Cohesin, a ring-shaped protein complex that wraps around sister chromatids is the molecular agent of sister chromatid cohesion, which persists from the time of DNA replication until anaphase. A distinct protein complex containing Scc2NIPBL and Scc4Mau2 (Scc2/4) initiates linkage of cohesin with DNA, and an in vitro reconstitution of cohesin loading by Scc2/4 suggests that the product of this reaction is a topological protein–DNA linkage. In addition to initiating a connection between cohesin and chromatin, Scc2/4 determines the timing and location of cohesin loading. We report here the structure of yeast Scc4 in complex with an N-terminal fragment of Scc2 and demonstrate that Scc4 determines cohesin localization through a conserved patch on its surface.

We obtained crystals of full-length Scc4 in complex with an N-terminal, 181-residue fragment of Scc2. We used an incomplete model, built into a 2.8 Å resolution map, to obtain phase information by molecular replacement for diffraction data from crystals of a native protein complex, extending to a minimum Bragg spacing of 2.1 Å. Scc4 is a superhelical array of 13 TPR modules with a beta ribbon insertion between repeats 6 and 7. Repeat 8, which has a particularly long first helix, lacks a second helix and has instead an extended segment with a disordered surface loop. This irregularity divides the solenoid into two subdomains, TPRN (Scc41–384) and TPRC (Scc4391–624). Residues 10–50 of Scc2 snake along the continuous inner cavity of Scc4 and emerge at both ends, with the N-terminus of Scc2 close to the C-terminus of Scc4. First, the concave surface of Scc4 is entirely enclosed, and Scc2 dissociation would therefore require either unfolding or proteolysis of Scc2 or Scc4. Second, residues 58–132 of Scc2 extend beyond the axial groove and make extensive contact with the external surface of Scc4. Several Scc2–Scc4 contacts on the external face of Scc4 are also conserved, including Scc2F86, which stacks onto Scc4Y40-Y41, and Scc2112–120, which forms a helix that fits over a hydrophobic surface on Scc4 TPRN. Mapping Scc4 sequence conservation onto our structure revealed a cluster of extremely conserved, solvent-facing residues, some of them invariant among all eukaryotes we examined. We found unaccounted-for electron density in this patch, into which we modeled a sulfate group.

> MKSSHHHHHHENLYFQSNAMENLGDKLSISQVYHLAQEYRDHAYSIANKIGSEEGLKQYYGLMNMSIQMFQLLKTKCTLSVLEDSKVTFEMVELLIQETYNFDLAELYISSLKERLQTHQSDTDLVEEIMRCEFLLLHDLPLMRDSKFHYKIALRNCNELVQYMVNLQDELYQNWASVFQYVGVMLCIKLKQHRRVKTSFHGLLSQCREKSQWKWFLNLCYVNYLLNERFPIPEDALQELRSTELHTVGPELYAWKLALEMVIQLCKDGNITDHLNEFKNFFDTNKQSLVTNEGKGCVIKIMPRIALKVELPMIFHYKELKNILLLLQSVSYIVNCYDEKGNFSRKFLPKVYSTTQKLIKNIAAGGVSMNELDSRIQTYKSILEFCEFYKVWEQTLLKGAVVTTESPKLGPSPGYVRLLQAMKVQFEGGGAVEEYTRLAQSGGTSSEVKMISLLNCYTVQAARVSRCSGDKQGELVEQCNKVWLQVEKLLQETDLQFNPIWECTVTILWLFSHFEPFSWNPLPCSDKQRAEYVSKLREFYSSNKFVAGEAVADNRFKLKKALLLQILVNYLGGRMLEHDLGEIYAISAKCFDMCRQQGGMRKVQYVIGIWHLMNCTVAMRGKDVALTNAKLEALVKQITSVKQ;> MKSSHHHHHHENLYFQSNAMSYPGKDKNIPGRIIEALEDLPLSYLVPKDGLAALVNAPMRVSLPFDKTIFTSADDGRDVNINVLGTANSTTSSIKNEAEKERLVFKRPSNFTSSANSVDYVPTNFLEGLSPLAQSVLSTHKGLNDSINIEKKSEIVSRPEAKHKLESVTSNAGNLSFNDNSSNKKTKTSTGVTMTQANLA5-(3,4-dichlorophenyl)furan-2-carboxylic acid | C11 H6 Cl2 O3 | 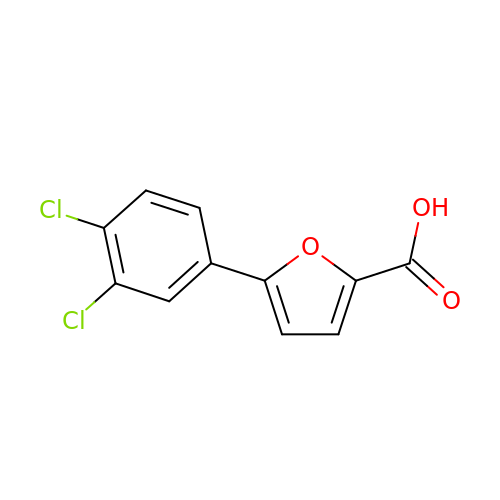GNXLBNMHCYYSPU-UHFFFAOYSA-N> MLVEHLRNFSESILESLETAIITLSKDGRITEWNKKAEQLFGLKKENVLGRRLKDLPDFEEIGSVAESVFENKEPVFLNFYKFGERYFNIRFSPFRNAKTQLLEGVIITIDDVTELYKYEEERKRRERLSILGEMTARVAHEIRNPITIIGGFIMRMKKHLDDPETLKKYINIITNELSRLETIVKEILEYSKERQVLEFTEFNLNELIREVYVLFEEKIRKMNIDFCFETDNEDLRVEADRTRIK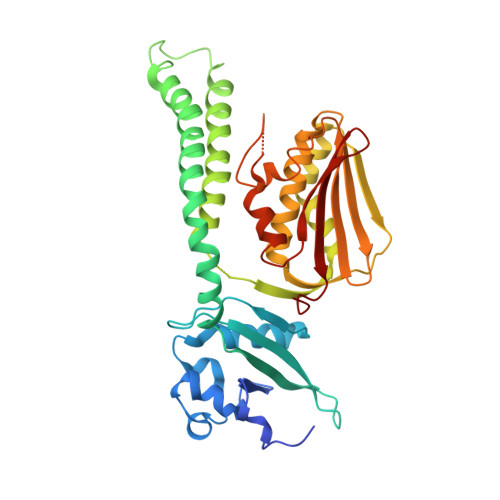QVLINLVQNAIEATGENGKIKITSEDMYTKVRVSVWNSGPPIPEELKEKIFSPFFTTKTQGTGLGLSICRKIIEDEHGGKIWTENRENGVVFIFEIPKTPEKR> MEINVTAPALLTDEHILQPFDCGNEVLSNWLRGRAMKNQMLNASRTFVICLEDTLRIVGYYSLATGSVTHAELGRSLRHNMPNPVPVVLLGRLAVDVCTRGH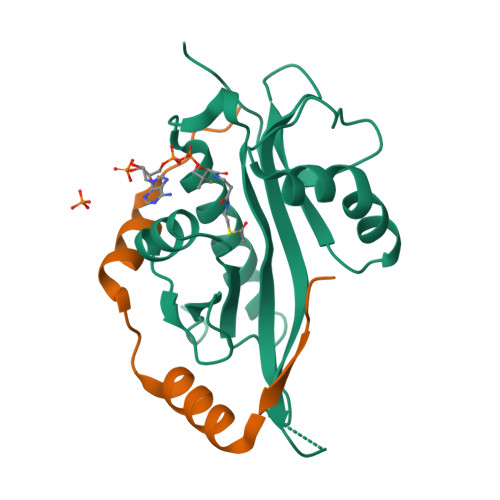GFGKWLLSDAIHRVVNLADQVGIKAVMVHAIDDDARAFYERFGFVQSVVAPNTLFYKVLEHHHHHH;> MASQRLFVLDNERYDSFITQLEAPVQNAEGRERLMAVKPEWK>QNNQTYANYSAQGQPDLYPETLATLTLSFPDCEHGPLKNNLVCDSSAGYVERAQALISLFTLEELILNTQNSGPGVPRLGLPNYQVWNEALHGLDRANFATKGGQFEWATSFPMPILTTAALNRTLIHQIADIISTQARAFSNSGRYGLDVYAPNVNGFRSPLWGRGQETPGEDAFFLSSAYTYEYITGIQGGVDPEHLKVAATVKHFAGYDLENWNNQSRLGFDAIITQQDLSEYYTPQFLAAARYAKSRSLMCAYNSVNGVPSCANSFFLQTLLRESWGFPEWGYVSSDCDAVYNVFNPHDYASNQSSAAASSLRAGTDIDCGQTYPWHLNESFVAGEVSRGEIERSVTRLYANLVRLGYFDKKNQYRSLGWKDVVKTDAWNISYEAAVEGIVLLKNDGTLPLSKKVRSIALIGPWANATTQMQGNYYGPAPYLISPLEAAKKAGYHVNFELGTEIAGNSTTGFAKAIAAAKKSDAIIYLGGIDNTIEQEGADRTDIAWPGNQLDLIKQLSEVGKPLVVLQMGGGQVDSSSLKSNKKVNSLVWGGYPGQSGGVALFDILSGKRAPAGRLVTTQYPAEYVHQFPQNDMNLRPDGKSNPGQTYIWYTGKPVYEFGSGLFYTTF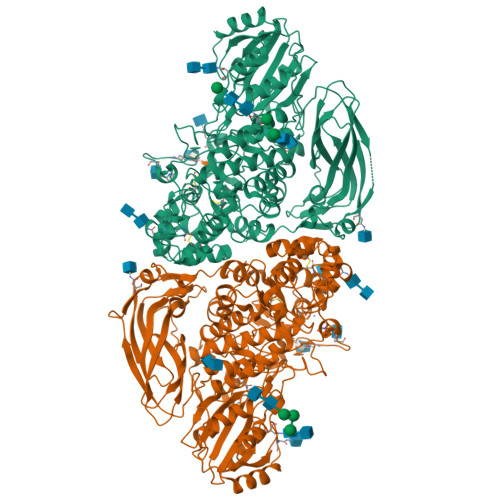KETLASHPKSLKFNTSSILSAPHPGYTYSEQIPVFTFEANIKNSGKTESPYTAMLFVRTSNAGPAPYPNKWLVGFDRLADIKPGHSSKLSIPIPVSALARVDSHGNRIVYPGKYELALNTDESVKLEFELVGEEVTIENWPLEE[2x]>MHAALSPLSQRFERIAVQPLTG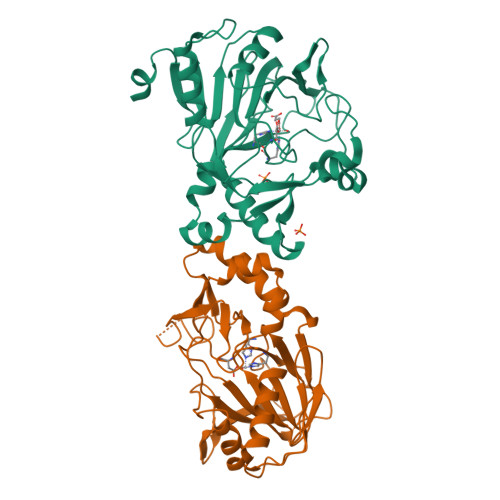VLGAEITGVDLREPLDDSTWNEILDAFHTYQVIYFPGQAITNEQHIAFSRRFGPVDPVPLLKSIEGYPEVQMIRREANESGRVIGDDWHTDSTFLDAPPAAVVMRAIDVPEHGGDTGFLSMYTAWETLSPTMQATIEGLNVVHSATRVFGSLYQAQNRRFSNTSVKVMDVDAGDRETVHPLVVTHPGSGRKGLYVNQVYCQRIEGMTDAESKPLLQFLYEHATRFDFTCRVRWKKDQVLVWDNLCTMHRAVPDYAGKFRYLTRTTVGGVRPAR[2x]> MPGAVEGPRWKQAEDIRDIYDFRDVLGTGAFSEVILAEDKRTQKLVAIKCIAKKALEGKEGSMENEIAVLHKIKHPNIVALDDIYESGGHLYLIMQLVSGGELFDRIVEKGFYTERDASRLIFQVLDAVKYLHDLGIV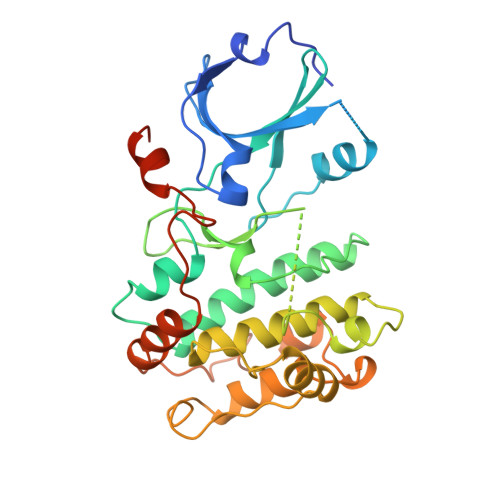HRDLKPENLLYYSLDEDSKIMISDFGLSKMEDPGSVLSTACGTPGYVAPEVLAQKPYSKAVDCWSIGVIAYILLCGYPPFYDENDAKLFEQILKAEYEFDSPYWDDISDSAKDFIRHLMEKDPEKRFTCEQALQHPWIAGDTALDKNIHQSVSEQIKKNFAKSKWKQAFNATAVVRHMRKLQLGHQPGGTGTDS[(1R)-2-cyclobutyl-1-({[(1R,2S,5S)-3-(N-{[(1S)-2,2-dimethyl-1-{[methyl(methylsulfonyl)amino]methyl}propyl]carbamoyl}-3-methyl-L-valyl)-6,6-dimethyl-3-azabicyclo[3.1.0]hex-2-yl]carbonyl}amino)ethyl]boronic acid | C29 H54 B 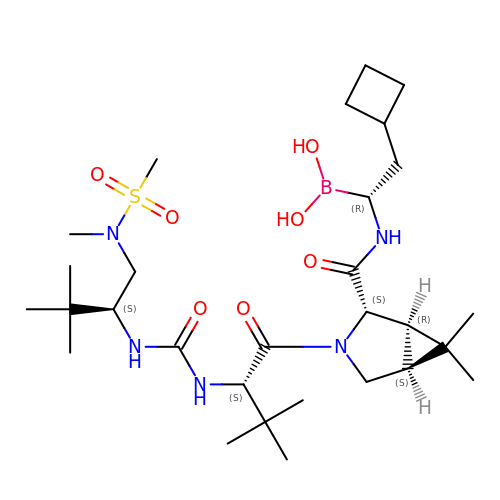N5 O7 S | KGZWDDBJGGJYLY-WKOLOUIMSA-N> MNHKVHHHHHHIEGAAMNEFARKKRALEHSRRINAGDLDAIIDLYAPDAVLEDPVGLPPVTGHDALRAHYEPLLAAHLREEAAEPVAGQDATHALIQISSVMDYLPVGPLYAERGWLKAPDAPGTARIHRTAMLVIRMDASGLIRHLKSYWGTSDLSGGSGPAADEAARKQMAVDYAERINAGDIEGVLDLFTDDIVFEDPVG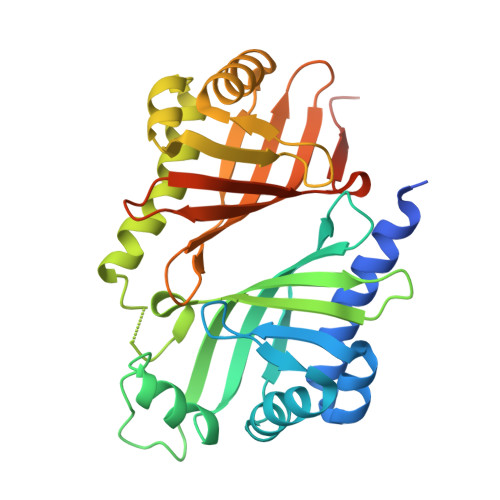RPPMVGKDDLRRHLELAVSCGTHEVPDPPMTSMDDRFVVTPTTVTVQRPRPMTFRIVGIVELDEHGLGRRVQAFWGVTDVTMDDRVQAFWGVTDVTMDD> MASNNYQPASSYIQPSFAGGELAPSLQGRVDLARYAISLKTCRNFVVQPYGGASNRPGFRFNTACKYKNYATRLIPFSFNTEQTYVIEIGHQYMRFHRDGAPVLDGGEPVEVATSWHRDDIFEIKYVQSADVLTLVHPDYKPRQLKRYSETDWVLDFFDNEFGPLQDQNVDESITIISNGVVDLVELTASEAIFSEAMVGTTIKLQQVSSGEVAAWQNRSAVEQGDLAYVDERTYKATSLSGGVDNTLTGD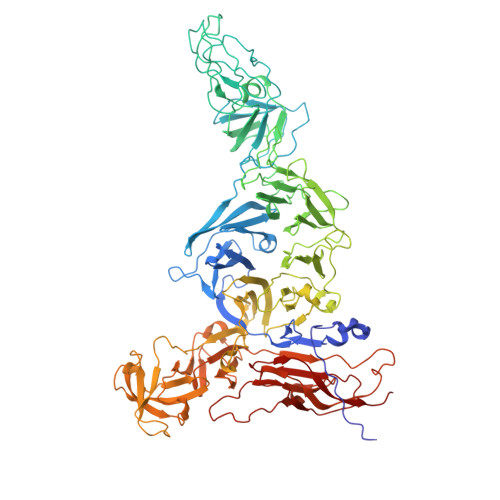NTPAHTEGEQWDGPRTTIQGVTETLGVKWAYLHSGFGYVRITEHRDDTHIVGRVIGRLPEEIRTEGTYRWSFAAWDSDRGYPGTASYYQQRLVFANSRAEPQAFWMSETGIFNGFKVSFPIEADDAITFTLASRQVNEIRHLIPLGSLLALTSGAEWMISDNDQGLAPDTVSADVQGYRGASDVTPLLIGSSALYVQARGTVIRDLAYSFELDGYTGDDLTIFSNHLLKDYTIKDWAYAQEPDSVVWLVRSDGALLSMTYQREQQVVAWARHDTVDGEFESVAVIAEGSRDVPYAIVKRQVGGETVRYIEYLDSRRFSHVEDFFCVDSGLTYDGRSSTGALLTIGGGTNWTTDEDLTLTASASSFSPSDVGRRVRVYTGDKFADVDVDAYVSATSVAVSAVRIVPEELRGVQGDRWGFMAKTLTGLDHLEGKTVSILADGNVHAPEVVTGGQVTLDYSAAVVHVGLPIESDIETLPISSSGATVRDSHKAIVGVGIQLEKSRGVFAARSRRDFTSSDLIELKQRDAEDWGEATGLETGLVELGIPTSWDKDGSLFIRQSDPLPLTILSIIPRVVMGGKG> GGSGSSKSSRLYDDYYNIPYQYSNPTPMNRDYNDVGSRINADKLVPEEYKRNTEFINKAVQQNKELNFKLREKQNEIFELKKIAETLRSKLEKYVDITKKLEDQNLNLQIKISDLEKKLSDANSALKLMQYIGDAIGTIRDPQELFRTVTDKLRLLFAFDSAVII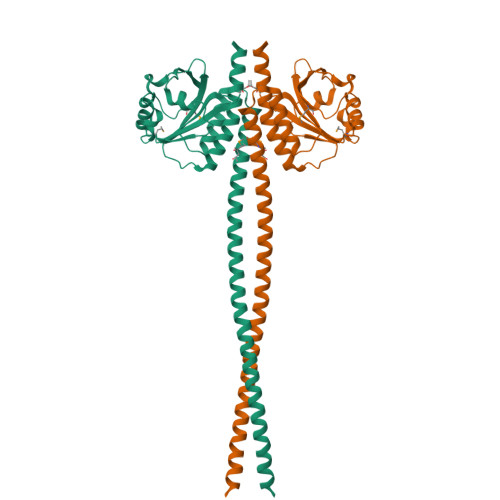TIDRERREASVFFEMLRFELPEQLRHQTRSIAGTWLEGHLDDRTVTVASIARDIPSFGADGAPLLWTLHELGMRQIVLSPLRSGGRVIGFLSFVSAEEKLWSDGDKSLLSGVSSSIAIAVSNALAYEALRQRE The direct activators of JNKs are the MAP2Ks MKK7 and MKK4.29 Targeting upstream kinases of MKK4/7 has been met with limited success due to possible activator redundancy, whereas targeting JNK itself has not shown clinical success yet, perhaps due to on-target toxicity. Thus, we considered the protein kinase MKK7, which exclusively phosphorylates JNK (whereas MKK4 also cross-talks with the p38 pathway) would be a prime target for selective JNK pathway inhibition. We have previously developed selective acrylamide inhibitors for MKK7 and set out to use them as starting points for optimization. We successfully determined six novel MKK7-ligand complexes with three members of each series: 1a, 1h, 1k and 2a, 2b, 2c.

Throughout series 1, the 4-amino-pyrazolopyrimidine core forms the expected hinge contacts to Glu213 and Met215, as well as a covalent bond between the piperidine-linked acrylamide and the thiol side chain of Cys218. The moieties introduced in the 3-position of the scaffold by CuAAC point toward the α-helix C and occupy the back pocket of the active binding site. In all three complexes, the enzyme is present in the active DFG-in conformation stabilized by the bound ligand, consistent with typical characteristics of type-I kinase inhibitors. However, the various substitutions of series 1 were able to make new productive interactions in the back pocket. Two common structural features were enriched in the top hits originating from derivatization of 1: halogenated hydroxyphenyls and phenethyl derivatives. All selected compounds derived from 1 showed a significant improvement in their inhibitory ability compared to the parent scaffold.

> MGHHHHHHSAKQTGYLTIGGQRYQAEINDLENLGEMGSGTCGQVWKMRFRKTGHVIAVKQMRRSGNKEENKRILMDLDVVLKSHDCPYIVQCFGTFITNTDVFIAMELMGTCAEKLKKRMQGPIPERILGKMTVAIVKALYYLKEKHGVIHRDVKPSNILLDERGQIKLCDFGISGRLVDSKAKTRSAGCAAYMAPERIDPPDPTKPDYDIRADVWSLGISLVELATGQFPYKNCKTDFEVLTKVLQEEPPLLPGHMGFSGDFQSFVKDCLTKDHRKRPKYNKLLEHSFIKRYETLEVDVASWFKDVMAKTRSPRTSG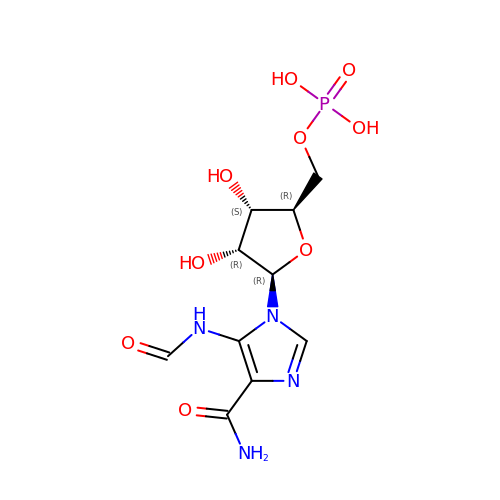5-(formylamino)-1-(5-O-phosphono-beta-D-ribofuranosyl)-1H-imidazole-4-carboxamide | C10 H15 N4 O9 P | ABCOOORLYAOBOZ-KQYNXXCUSA-N Here we show that these genes encode a Ni2+-dependent enzyme that efficiently and specifically hydrolyzes metformin to guanylurea and dimethylamine. The active enzyme is a heteromeric complex of α- and β- subunits in which only the α-subunits contain the conserved His and Asp residues for the coordination of two Ni2+ ions in the active site. A crystal structure of metformin hydrolase reveals an α2β4 stoichiometry of the hexameric complex, which is unprecedented in the ureohydrolase family. Our findings establish the molecular basis for metformin hydrolysis to guanylurea as the primary pathway for metformin biodegradation and provide insight into the recent evolution of ureohydrolase family proteins in response to an anthropogenic compound.

For crystallization, we used AnMefH as it shares a higher sequence identity with DmgH than PmMefH (93.5% and 93.3% sequence identity for the alpha subunits, respectively), so that residues responsible for the change in substrate specificity are easier to identify. The best diffraction data was obtained from AnMefH crystals that were soaked with urea prior to vitrification and X-ray analysis. In the obtained structure, both MefHα and MefHβ adopt an almost identical three-layer alpha-beta-alpha fold typical for members of the ureohydrolase family, but diverge notably at the N-terminal loop regions that are distinct to each subunit type. The global structure of MefH is distinct amongst ureohydrolase family proteins since it is a heterohexamer consisting of a dimer of heterotrimers, each with αβ2 stoichiometry. The MefHα subunits are located in apical position and make a close contact between both trimers. In contrast, the MefHβ subunits interact weakly with their counterparts in the opposite trimer. Each MefHα subunit coordinates two metal ions in its active site through four Asp (D183, D187, D276 and D278) and two His (H158 and H185) residues. The electron density in the active site is best explained by two Ni2+ ions, which is in agreement with the ICP-OES experiments and the metal dependency of the enzyme. In the crystal structure, the Ni2+ ions coordinate a molecule of urea. In contrast, the corresponding region of the MefHβ subunits do not contain any metal ions or ligands, and four of the six residues that bind Ni2+ in the MefHα subunits are replaced by amino acids that are not prone to coordinate cations.

>[4x]MNPAKSYAHLFSPLGGDAGDNYRAPGLITFLRSAHVPLNAEALKACGAKYAFVGVPFDEGNIGKPGSEDAPREFRLITQEYFSYWFEYNVDLHGKAVDCGDVSMPKVSPEVAHERIYRAVREVLKSGLIPIICGGDRSISITAARALSDHIGPQKKMGYMHFGAQLDMADSWAGERNLAPCAMARITELPNLDIRNVAHLGARNAMNPKDHIDLSKERGLQYDSMFDLFDAGIYPLVERSIDRVWSGTDAQYLGFNFNVMDSSTAPGVTSTEPGGLESREMMRIVDMIAKRGGVSVIDLTELCPIFDISGTAARLAACVIMRLMASLAAQDGDVIDDKLRRTDLVAAE;>MAWSHPQFEKVENLYFQGAMLDRKTETAKWQFTPHQHRGPAEQFGENDHIYSPKLHNGSFKSRGLATFMGAPYCPPDRHKIREMGAKICFLAVPWDQGQIVRAGASQGAAGLRDATTQYFPYMFEYDVDLLSFFRVVDCGDVPTVPGNNIKSQEYTADYVTECLEGGAKVILFGGDHSLPIPGAKALSRFTGSGKMGYLHVDCHLDAGPDWAGNLITNCSGAPRALDLPNCNARNMAHMGSRNSLNPKDWWDFYVDNEIRVVTMPEMIERGLEVCANEIFERVKKDTDSLYFTWDTDSIDISCMPANSAPECYGLKGREVIQLARIAGRHGCDILDIVELCPDFDPSQISVKMTVNMIYHYLGSRAQTLRQQGKQP[2x]(1-methylcyclopropyl)methyl 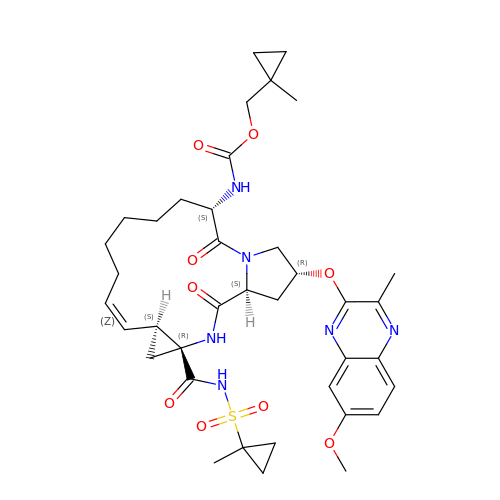{(2R,4S,6S,12Z,13aS,14aR,16aS)-2-[(7-methoxy-3-methylquinoxalin-2-yl)oxy]-14a-[(1-methylcyclopropane-1-sulfonyl)carbamoyl]-5,16-dioxo-1,2,3,5,6,7,8,9,10,11,13a,14,14a,15,16,16a-hexadecahydrocyclopropa[e]pyrrolo[1,2-a][1,4]diazacyclopentadecin-6-yl}carbamate | C38 H50 N6 O9 S | FVAHUZNNBVVCMP-ZJYMAAHDSA-N>MSTLAEVYTIIEDAEQECRKGDFTNAKAKYQEAIEVLGPQNENLSQNKLSSDVTQAIDLLKQDITAKIQELELLIEKQSSEENNIGMVNNNMLIGSVILNNKSPINGISNARNWDNPAYQDTLSPINDPLLMSILNRLQFNLNNDIQLKTEGGKNSKNSEMKINLRLEQFKKELVLYEQKKFKEYGMKIDEITKENKKLANEIGR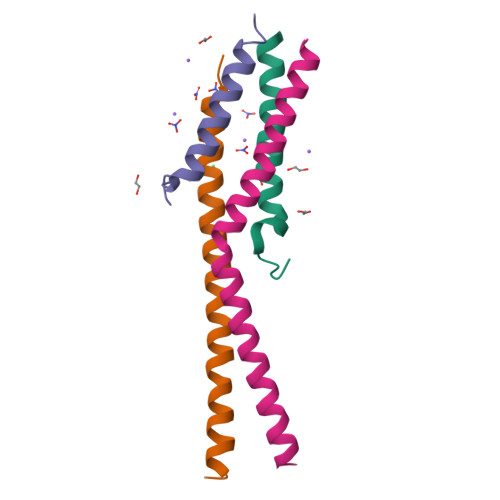LRERWDSLVESAKQRRDKQKN[12x]>SVRSSSRTPSDKPVAHVVANPQAEGQLQWLNRRANALLANGVELRDNQLVVPSEGLYLIYSQVLFKGQGCPSTHVLLTH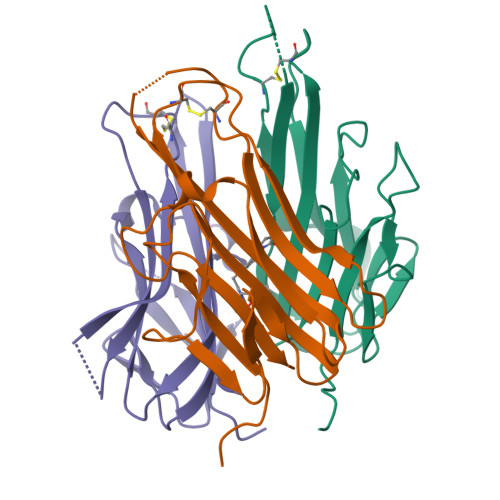TISRIAVSYQTKVNLLSAIKSPCQRETPEGAEAKPWYEPIYLGGVFQLEKGDRLSAEINRPDYLDFAESGQVYFGIIAL[3x]>GAILAARIAVSNLHKETKKVFSDVMEDLYNYINPHNGKHSPMVAKSTLDIVLANKDRLNSAIIYDRDFSYNYFGFKTLERSYLLKINGKVAERPQHMLMRVSVGIHKEDIDAAIETYNLLSERWFTHASPTLFNAGTNRPQLSSCFLLSMKDDSIEGIYDTLKQCALISKSAGGIGVAVSCIRATGSYIAGTNGNSNGLVPMLRVYNNTARYVDQGGNKRPGAFAIYLEPWHLDIFEFLDLKKNTGKEEQRARDLFFALWIPDLFMKRVETNQDWSLMCPNECPGLDEVWGEEFEKLYASYEKQGRVRKVVKAQQLWYAIIESQTETGTPYMLYKDSCNRKSNQQNLGTIKCSNLCTEIVEYTSKDEVAVCNLASLALNMYVTSEHTYDFKKLAEVTKVVVRNLNKIIDINYYPVPEACLSNKRHRPIGIGVQGLADAFILMRYPFESAEAQLLNKQIFETIYYGALEASCDLAKEQGPYETYEGSPVSKGILQYDMWNVTPTDLWDWKVLKEKIAKYGIRNSLLIAPMPTASTAQILGNNESIEPYTSNIYTRRVLSGEFQIVNPHLLKDLTERGLWH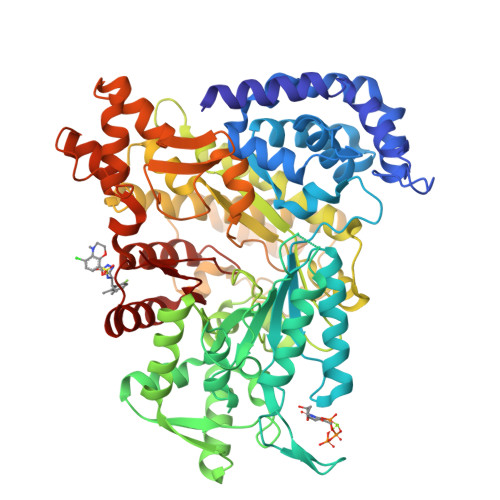EEMKNQIIACNGSIQSIPEIPDDLKQLYKTVWEISQKTVLKMAAERGAFIDQSQSLNIHIAEPNYGKLTSMHFYGWKQGLKTGMYYLRTR[2x]>KVNQNQAKRCTVIGGSGFLGQHMVEQLLARGYAVNVFDIQQGFDNPQVRFFLGDLCSRQDLYPALKGVNTVFHCASPPPSSNNKELFYRVNYIGTKNVIETCKEAGVQKLILTSSASVIFEGVDIKNGTEDLPYAMKPIDYYTETKILQ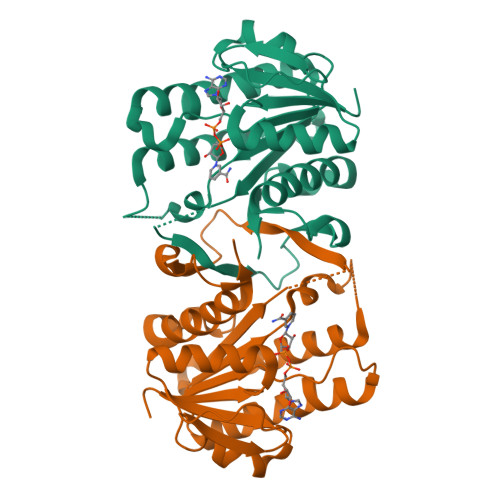ERAVLGANDPEKNFLTTAIRPHGIFGPRDPQLVPILIEAARNGKMKFVIGNGKNLVDFTFVENVVHGHILAAEQLSRDSTLGGKAFHILEHHHHHH[2x]> MSFINYSSREINCKIVYYGPGLCGKTTNLQYIYNKTAAETKGKLISLSTETDRTLFFDFLPLSLGEIRGFKTRFHLYTVPGQVFYDASRKLILKGVDGVVFVADSQIERMEANMESLENLRINLAEQGYDLNKIPYVIQYNKRDLPNAVTVEEMRKALNHRNIPEYQAVAPTGVGVFDTLKAVAKLVLTELKKGGGSHHHHHH;>MGTQLVMYEEEFTKINAVCDRLTKDANAKVVFLVDKNGQLISSAGQTQNIDTTSLASLTAGNVAAMGGLAKLIGENEFPNQFHEGAKDSLYMTIVGSRVVLVVIFDNRTSLGLVRLRIKKASDELTKIFESLVKKTDSPGAGSPFAEMSDDDIDNLFSEGSHHHHHH[2x]

The localization of motility complexes, and thereby the direction of movement, is determined by an oscillatory system, which includes Mutual gliding motility A (MglA), a small Ras-like GTPase, and Mutual gliding motility B (MglB), its GTPase activating protein (GAP) as major components. In this study, we report the biochemical and structural characterization of M. xanthus MglA and MglB (MxMglA and MxMglB). Thus, MxMglB plays a dual role in increasing the GTPase activity of MxMglA by orienting the catalytic residues (role of a GAP) and by facilitating exchange of GDP with GTP (role of a GEF). Allosteric binding of the C-terminal helix (Ct-helix) of MxMglB on MxMglA facilitates nucleotide exchange.

In the structure, a monomer of MxMglA was bound to a dimer of MxMglB. MxMglA interacts with the MxMglB dimer through an extensive hydrophobic interface involving β2 strand of MxMglA and α2 helices of MxMglB monomers, an interface similar to that of TtMglAB. One of the novel features of the MxMglAB–GTPγS complex is the asymmetry between the 2 protomers of MxMglB (labeled MglB1 and MglB2). In MglB1, the N-terminal amino acids (2–7) comprised a β-strand that formed hydrogen bonds with the β0 strand of MxMglA, thus continuing the central β-sheet of the MxMglA fold. α1 helix of the Rbl/LC7 fold started from Glu11B (residue names with superscript B denote residues of MglB) of MglB1. However, residues 147 to 157 of the MglB1 protomer could be modeled into the electron density, which adopted a helical conformation. Henceforth, this will be referred to as Ct-helix (C-terminal helix of MxMglB). The Ct-helix of MglB1 bound to a pocket in MxMglA distal from the nucleotide-binding site. The binding pocket in MxMglA was formed by the residues of the α5 helix, β2 strand, and the loop connecting β2 and β3 strands (β2–β3 loop) of MxMglA (interswitch region of small Ras-like GTPases). The conformational changes between MxMglA–GDP and the MxMglA–GTPγS bound to MxMglB resulted in movements of switch 1 and switch 2 such that Arg53A and Gln82A of MxMglA are now oriented towards the catalytic water. Analysis of the crystal structure of MxMglAB–GTPγS complex showed that Asp150B, Asp151B, and Asp152B on the MxMglB Ct-helix formed water-mediated as well as direct interactions with MxMglA.> 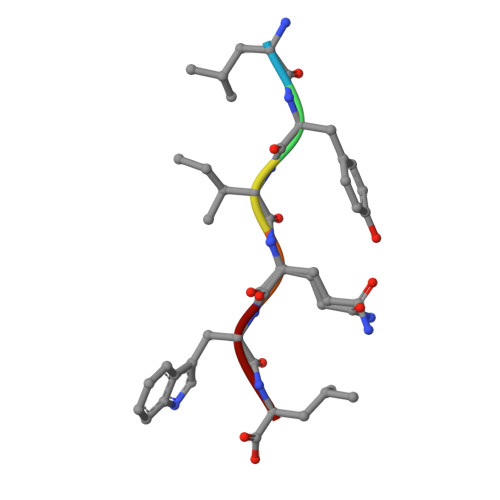LYIQWL>GSHMRKIQRYVRKDGKCNVHHGNVRE[2x];>KRAETLVFSTHAVISMRDGKLCLMFRVGDLRNSHIVEASIRAKLIKSKQTSEG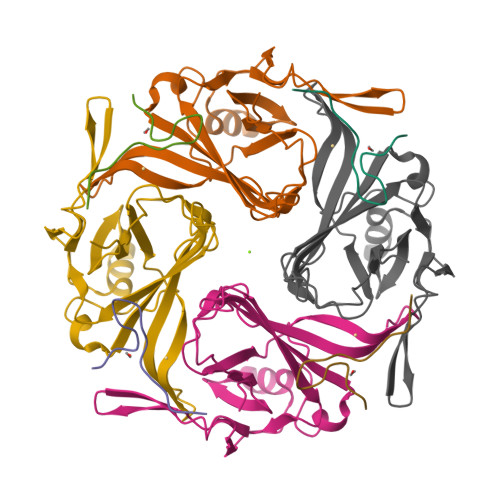EFIPLNQTDINVGYYTGDDRLFLVSPLIISHEINQQSPFWEISKAQLPKEELEIVVILEGMVEATGMTCQARSSYITSEILWGYRFTPVLTLEDGFYEVDYNSFHETYETSTPSLSAKELAELANRAEL[2x]>[8x]MAKNTSITLGEHFDGFITSQIQSGRYG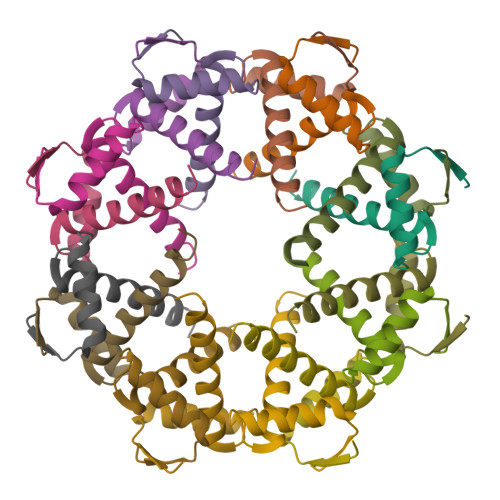SASEVIRSALRLLENQETKLQSLRQLLIEGEQSGDADYDLDSFINELDSENIR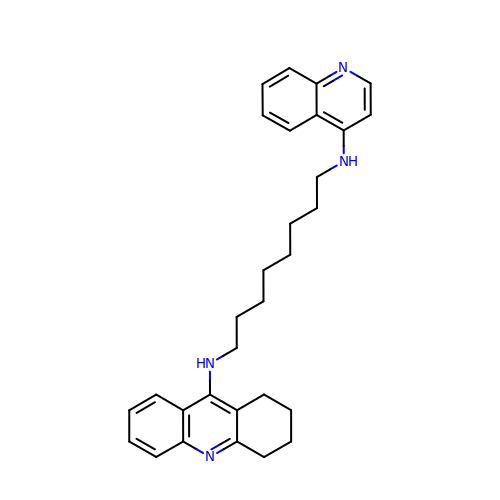N-QUINOLIN-4-YL-N'-(1,2,3,4-TETRAHYDROACRIDIN-9-YL)OCTANE-1,8-DIAMINE | C30 H36 N4 | UNVOAAWEEGAXTN-UHFFFAOYSA-N> MDREPQHEELPGLDSQWRQ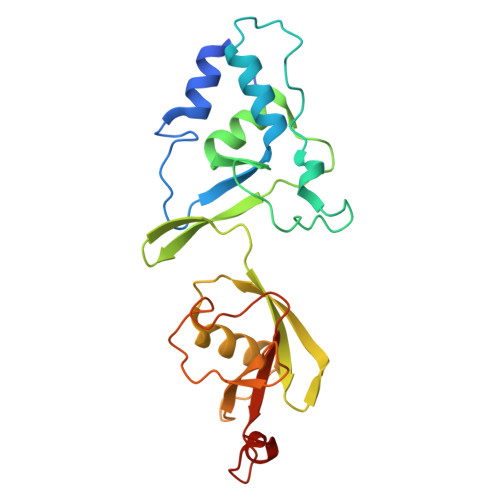IENGESGRERPLRAGESWFLVEKHWYKQWEAYVQGGDQDSSTFPGCINNATLFQDEINWRLKEGLVEGEDYVLLPAAAWHYLVSWYGLEHGQPPIERKVIELPNIQKVEVYPVELLLVRHNDLGKSHTVQFSHTDSIGLVLRTARERFLVEPQEDTRLWAKNSEGSLDRLYDTHITVLDAALETGQLIIMETRKKDGTWPSAQLEHHHHHH>[2x]MAMTVTEVDLPPIYCPLESAIHP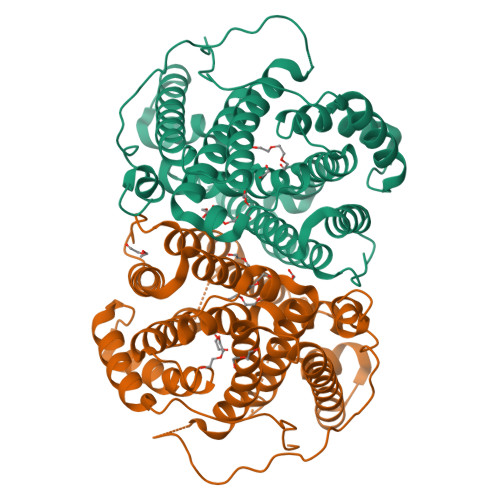RVHEVEKRAVEWIRRSGMCASEEERAWVIATHSADFFARFAPTAADEDRLLATSLWVYWGFAFDDHRCDNGPLSTRPAQFNALAGRVQRALEAPSAEDNGDRFVPALQDIARRFRSFGTPTQVRRFVHAHRAWLSGVAWQIGNQARGHMPGLDDYLAMRLLSAGGEPTFAMLEIATGAEVPAQDLERPAVRALTEMAIMVAALDNDRHSLRKELSRGHTDQNIYSVLMHHRGMSLQEAVEEATKLRDRILLRFLELHDRVRPGAGAELSTYLQGLRHGIRGNAEWGLRVPRYLSLGRVPDPMEDAPLTWAESPSDSSPSPLPGAPSIAWWWDDALLGA>GSMQPDMSLNVIKMKSSDFLESAELDSGGFGKVSLAFHRTQGLMIMKTVYKGPNCIEHNEALLEEAKMMNRLRHSRVVKLLGVIIEEGKYSLVMEYMEKGNLMHVLKAEMSTPLSVKGRIILEIIEGMAYLHGKGVIHKDLKPENILVDNDFHIKIADLGLASFKMWSKLNNEEHNELREVDGTAKKNGGTLYYMAPEHLNDVNAKPTEKSDVYSF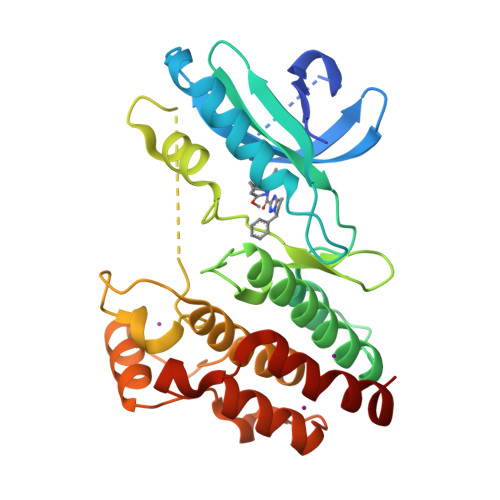AVVLWAIFANKEPYENAIAEQQLIMAIKSGNRPDVDDITEYCPREIISLMKLCWEANPEARPTFPGIEEKFRPFYLSQLE[2x]>[2x]MAHHHHHHVDDDDKMLVPRGSENLYFQGSAMDPPTFTFNFNNEPWVRGRHETYLCFTMEVVKHHSPVSWKRGVFRNQVDPETHCHAERCFLSWFCDDILSPN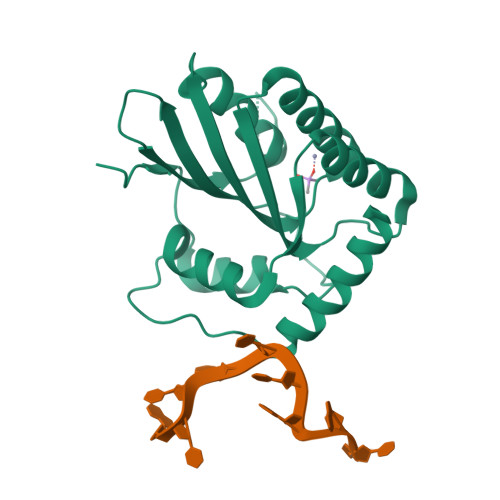TNYEVTWYTSWSPCPECAGEVAEFLARHSNVNLTIFTARLYYFWDTDYQEGLRSLSQEGASVEIMGYKDFKYCWENFVYNDDEPFKPWKGLKYNFLFLDSKLQEILE> AKYTRGTVTAFSPFDARADAEALRKAMKGMGTDEETILKILTSRNNAQRQEIASAFKTLFGRDLVDDLKSELTGKFETLMVSLMRPARIFDAHALKHAIKGAGTNEKVLTEILASRTPAEVQNIKQVYMQEYEANLEDKITGETSGHFQRLLVVLLQANRDPDGRVDEALVEKDAQVLFRAGELKWGTDEETFITILGTRSVSHLRRVFDKYMTISGFQIEETIDRETSGDLEKLLLAVVKCIRSVPAYFAETLYYSMKGAGTDDDTLIRVMVSRSEIDLLDIRH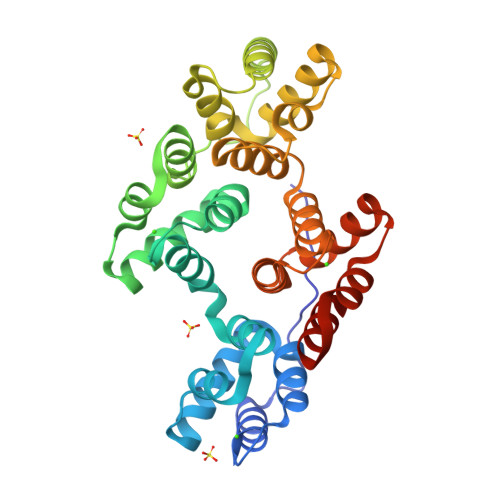EFRKNFAKSLYQMIQKDTSGDYRKALLLLCGGDDE pmcThe enzyme 2′-deoxynucleoside 5′-phosphate N-hydrolase 1 (DNPH1) (EC 3.2.2.-) is responsible for catabolizing toxic 5-hydroxymethyl-2′-deoxyuridine 5′-monophosphate (5hmdUMP), a noncanonical 2′-deoxynucleotide that, if incorporated into DNA, must be excised via DNA repair pathways. DNPH1 catalyzes the hydrolysis of the N-ribosidic bond of 2′-deoxynucleoside 5′-monophosphates to produce 2-deoxyribose 5-phosphate and the corresponding nucleobase.5HsDNPH1 also accepts canonical 2′-deoxynucleoside 5′-monophosphates as substrates, albeit with very low reaction rates. The dimeric form is common for DNPH1 and is essential for catalysis. The overall fold is similar to previously reported inhibitor-bound structures of HsDNPH1 and rat DNPH1,6−8 with a five-stranded parallel β-sheet core surrounded by five α-helices.

To investigate the structural basis for catalysis of N-ribosidic bond cleavage, the structures of unbound HsDNPH1Trunc and dUMP-bound complex were solved with data to 1.7 and 1.42 Å resolution, respectively. Unliganded HsDNPH1Trunc and dUMP complex structures have four and two molecules in the asymmetric unit, comprising two dimers and one dimer, respectively. Buried surface areas were calculated by PISA24 analysis to be 1241.0 and 1267.5 Å2 for unbound and substrate-bound dimers, respectively. Binding of dUMP stabilizes the Ile29–Glu34 loop, for which no electron density can be seen in the absence of the substrate, probably as a result of high flexibility. Overlay of the unliganded and Michaelis complex structures yielded a small root-mean-square deviation of 0.52 Å over 117 Cα atoms. An intriguing feature of the HsDNPH1Trunc crystal structures is the presence of an apparent low-barrier hydrogen bond (LBHB) between the −COO– and −OH groups of the highly conserved residues Glu104 and Tyr24 as inferred from the O–O distances in unbound HsDNPH1Trunc and HsDNPH1Trunc:dUMP complexes, respectively. The distance between the O atoms of the Glu104 −COO– and Tyr24 −OH groups is 2.3 Å in the unbound and 2.4 Å in the dUMP-bound enzyme. As the Glu residue in the equivalent position to Glu104 is proposed to act as a nucleophile in the rat DNPH1,10 the apparent LBHB might be involved in tuning the position and nucleophilicity of Glu104 in HsDNPH1. The small increase in the apparent LBHB length in the Michaelis complex as compared with the unliganded enzyme, still insufficient to disrupt the apparent LBHB, might reflect the poor substrate nature of the dUMP (kcat/KM of 27 M–1 s–1).

>[4x]GMRPALYFCGSIRGGREDRTLYERIVSRLRRFGTVLTEHVAAAELGARGEEAAGGDRLIHEQDLEWLQQADVVVAEVTQPSLGVGYELGRAVAFNKRILCLFRPQSGRVLSAMIRGAADGSRFQVWDYEEGEVEALLDRYFEADP>MELIRIAMKKDLENDNSLMNKWATVAGLKNPNPLYDFLNHDGKTFNEFSSIVNIVKSQYPDREYELMKDYCLNLDVKTKAARSALEYADANMFFEIEDALIDSMISCSNMKSKEYGKVYKIHRELSKGEIDVFEASANIGKQRIKTAEMNIFSKMLLMYDCLNKGNFAPMMLLFQQIDLSEIKENRYLKNSFETRINVLLSNIYLNENNLELCREYAQKAISSTDTQRFLVFSYLTIGTSYIFSDFNLSKQNYLIGLKFAKGNPGFEEFFKRNLSFLNNFWNKENEWINYDSDAVTDMQEVIFELINHKELSKALQLLNKLEERDQNENELGFHYYLKGLITNEKEAFFKSVEYFKASQDKLSIKMPLIQLEKMGENPRLLKIITM[2x]

The arbitrium system is employed by phages of the SPbeta family to communicate with their progeny during infection to decide either to follow the lytic or the lysogenic cycle. The system is controlled by a peptide, AimP, that binds to the regulator AimR, inhibiting its DNA-binding activity and expression of aimX. AimR is a transcription factor that in its apo peptide-free form promotes aimX expression. In this study, we deepen our understanding of the system by solving the structure of an additional AimR that shows chimerical characteristics with the SPβ receptor.

In order to validate our proposed mechanism of action, we solved the crystal structure of AimRKat in complex with a 45 bp DNA fragment (AimRKat-DNA) which includes the aimX-boxKat with the two 6 bp inverted repeats recognised by DBD domain (identical to the ones recognised by AimRSPβ) and a 25 bp spacer. AimRKat-DNA crystals belong to space group P21 and diffracted to a resolution of 2.5 Å. The AimRKat-DNA asymmetric unit contains two AimR molecules arranged as a dimer and one duplex aimX-boxKat molecule. Overall, the structure is similar to AimRSPβ-DNA (RMSD ~2.1 Å), however, RMSD differences are not constant throughout the entire molecule. RMSD differences are minimal in the N-terminal part, which is bound to the DNA, and increase towards the C-terminal domain. As could be anticipated from the sequence identity between AimRKat and AimRSPβ (almost 100% for DBD, TPR1 and TPR2) and the identical inverted repeats in their target DNA boxes, both proteins bind to DNA using equivalent interactions. The α3 helix from DBD inserts into DNA major groove allowing specific DNA readout by side chains from residues N30, N32 and Y35 that interact with the T6C7A8/A36G37T38 portion from the ATCACT inverted repeat of aimX-boxKat. In addition, DNA binding is stabilised by an extensive indirect readout of the DNA backbone at both the inverted repeats and the spacer region. Meanwhile residues located in TPRN-ter are involved in the 25 bp spacer binding by mainly polar interactions. The high A-T content in the 25 bp spacer allows a small DNA bending of around 20° towards AimR interacting surface.>[2x]SNASSPSSPADWAKKLTDAVLRQKAGETLTAADRDFSNADFRNITFSKILPPSFMERDGDIIKGFNFSNSKFTYSDISHLHFDECRFTYSTLSDVVCSNTKFSNSDMNEVFLQYSITTQQQPSFIDTTLKNTLIRHKANLSGVILNEPDNSSPPSVSGGGNFIRLGDIWLQMPLLWTENAVDGFLNHEHNNGKSILMTIDSLPDKYSQEKVQAMEDLVKSLRGGRLTEACIRPVESSLVSVLAHPPYTQSALISEWLGPVQERFFAHQCQTYNDVPLPAPDTYYQQRILPVLLDSFDRNSAAMTTHSGLFNQVILHCMTGVDCTDGTRQKAAALY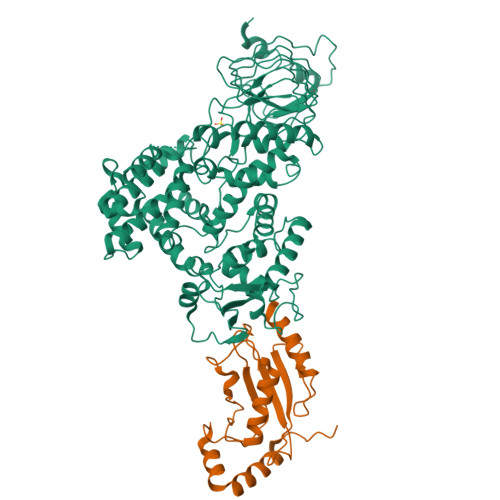EQYLAHPAVSPHIHNGLFGNYDGSPDWTTRAADNFLLLSSQDSDTAMMLSTDTLLTMLNPTPDTAWDNFYLLRAGENVSTAQISPVELFRHDFPVFLAAFNQQATQRRFGELIDIILSTEEHGELNQQFLAATNQKHSTVKLIDDASVSRLATIFDPLLPEGKLSPAHYQHILSAYHLTDATPQKQAETLFCLSTAFARYSSSAIFGTEHDSPPALRGYAEALMQKAWELSPAIFPSSEQFTEWSDRFHGLHGAFTCTSVVADSMQRHARKYFPSVLSSILPLAWA;>[2x]GSMAASRRLMKELEEIRKCGMKNFRNIQVDEANLLTWQGLIVPDNPPYDKGAFRIEINFPAEYPFKPPKITFKTKIYHPNIDEKGQVCLPVISAENWKPATKTDQVIQSLIALVNDPQPEHPLRADLAEEYSKDRKKFCKNAEEFTKKYGEKRPVD>SVTEFLKPRLVDIEQVSSTHAKVTLEPLERGFGHTLGNALRRILLSSMPGCAVTEVEIDGVLHEYSTKEGVQEDILEILLNLKGLAVRVQGKDEVILTLNKSGIGPVTAADITHDGDVEIVKPQHVICHLTDENASISMRIKVQRGRGYVPASTRIHSEEDERPIGRLLVDACYSPVERIAYNVEAARVEQRTDLDKLVIEMETNGTIDPEEAIRRAATILAEQLEAFVDLRDVRQPEVKEEKPEFDPILLRPVDDLELTVRSANCLKAEAIHYIGDLVQRTEVELLKTPNLGKKSLTEIKDVLASRGLSLGMRLENWPPA[2x];> MVYSYTEKKRIRKDFGKRPQVLDVPYLLSIQLDSFQKFIEQDPEGQYGLEAAFRSVFPIQSYSGNSELQYVSYRLGEPVFDVQECQIRGVTYSAPLRVKLRLVIYEREAPEGTVKDIKEQEVYMGEIPLMTDNGTFVINGTERVIVSQLHRSPGVFFDSDKGKTHSSGKVLYNARIIPYRGSWLDFEFDPKDNLFVRIDRRRKLPATIILRALNYTTEQILDLFFEKVIFEIRDNKLQMELVPERLRGETASFDIEANGKVYVEKGRRITARHIRQLEKDDVKLIEVPVEYIAGKVVAKDYIDESTGELICAANMELSLDLLAKLSQSGHKRIETLFTNDLDHGPYISETLRVDPTNDRLSALVEIYRMMRPGEPPTREAAESLFENLFFSEDRYDLSAVGRMKFNRSLLREEIEGSGILSKDDIIDVMKKLIDIRNGKGEVDDIDHLGNRRIRSVGEMAENQFRVGLVRVERAVKERLSLGDLDTLMPQDMINAKPISAAVKEFFGSSQLSQFMDQNNPLSEITHKRRISALGPGGLTRERAGFEVRDVHPTHYGRVCPIETPEGPNIGLINSLSVYAQTNEYGFLETPYRKVTDGVVTDEIHYLSAIEEGNYVIAQANSNLDEEGHFVEDLVTCRSKGESSLFSRDQVDYMDVSTQQVVSVGASLIPFLEHDDANRALMGANMQRQAVPTLRADKPLVGTGMERAVAVDSGVTAVAKRGGVVQYVDASRIVIKVNEDEMYPGEAGIDIYNLTKYTRSNQNTCINQMPCVSLGEPVERGDVLADGPSTDLGELALGQNMRVAFMPWNGYNFEDSILVSERVVQEDRFTTIHIQELACVSRDTKLGPEEITADIPNVGEAALSKLDESGIVYIGAEVTGGDILVGKVTPKGETQLTPEEKLLRAIFGEKASDVKDSSLRVPNGVSGTVIDVQVFTRDGVEKDKRALEIEEMQLKQAKKDLSEELQILEAGLFSRIRAVLVAGGVEAEKLDKLPRDRWLELGLTDEEKQNQLEQLAEQYDELKHEFEKKLEAKRRKITQGDDLAPGVLKIVKVYLAVKRRIQPGDKMAGRHGNKGVISKINPIEDMPYDENGTPVDIVLNPLGVPSRMNIGQILETHLGMAAKGIGDKINAMLKQQQEVAKLREFIQRAYDLGADVRQKVDLSTFSDEEVMRLAENLRKGMPIATPVFDGAKEAEIKELLKLGDLPTSGQIRLYDGRTGEQFERPVTVGYMYMLKLNHLVDDKMHARSTGSYSLVTQQPLGGKAQFGGQRFGEMEVWALEAYGAAYTLQEMLTVKSDDVNGRTKMYKNIVDGNHQMEPGMPESFNVLLKEIRSLGINIELED;> LLKFLKAQTKTEEFDAIKIALASPDMIRSWSFGEVKKPETINYRTFKPERDGLFCARIFGPVKDYECLCGKYKRLKHRGVICEKCGVEVTQTKVRRERMGHIELASPTAHIWFLKSLPSRIGLLLDMPLRDIERVLYFESYVVIEGGMTNLERQQILTEEQYLDALEEFGDEFDAKMGAEAIQALLKSMDLEQECEQLREELNETNSETKRKKLTKRIKLLEAFVQSGNKPEWMILTVLPVLPPDLRPLVPLDGGRFATSDLNDLYRRVINRNNRLKRLLDLAAPDIIVRNEKRMLQEAVDALLDNGRRGRAITGSNKRPLKSLADMIKGKQGRFRQNLLGKRVDYSGRSVITVGPYLRLHQCGLPKKMALELFKPFIYGKLELRGLATTIKAAKKMVEREEAVVWDILDEVIREHPVLLNRAPTLHRLGIQAFEPVLIEGKAIQLHPLVCAAYNADFDGDQMAVHVPLTLEAQLEARALMMSTNNILSPANGEPIIVPSQDVVLGLYYMTRDCVNAKGEGMVLTGPKEAERLYRSGLASLHARVKVRITEYEKDANGELVAKTSLKDTTVGRAILWMIVPKGLPYSIVNQALGKKAISKMLNTCYRILGLKPTVIFADQIMYTGFAYAARSGASVGIDDMVIPEKKHEIISEAEAEVAEIQEQFQSGLVTAGERYNKVIDIWAAANDRVSKAMMDNLQTETVINRDGQEEKQVSFNSIYMMADSGARGSAAQIRQLAGMRGLMAKPDGSIIETPITANFREGLNVLQYFISTHGARKGLADTALKTANSGYLTRRLVDVAQDLVVTEDDCGTHEGIMMTPVIEGGDVKEPLRDRVLGRVTAEDVLKPGTADILVPRNTLLHEQWCDLLEENSVDAVKVRSVVSCDTDFGVCAHCYGRDLARGHIINKGEAIGVIAAQSIGEPGTQLTMRTFHIGGAASRAAAESSIQVKNKGSIKLSNVKSVVNSSGKLVITSRNTELKLIDEFGRTKESYKVPYGAVLAKGDGEQVAGGETVANWDPHTMPVITEVSGFVRFTDMIDGQTITRQTDELTGLSSLVVLDSAERTAGGKDLRPALKIVDAQGNDVLIPGTDMPAQYFLPGKAIVQLEDGVQISSGDTLARIPQESGGTKDITGGLPRVADLFEARRPKEPAILAEISGIVSFGKETKGKRRLVITPVDGSDPYEEMIPKWRQLNVFEGERVERGDVISDGPEAPHDILRLRGVHAVTRYIVNEVQDVYRLQGVKINDKHIEVIVRQMLRKATIVNAGSSDFLEGEQVEYSRVKIANRELEANGKVGATYSRDLLGITKASLATESFISAASFQETTRVLTEAAVAGKRDELRGLKENVIVGRLIPAGTGYAYHQDRMRRRAAG;> ARVTVQDAVEKIGNRFDLVLVAARRARQMQVGGKDPLVPEENDKTTVIALREIEEGLINNQILDVRERQEQQEQ;> AGTPSGNGVGETTQSLQDYLMWQVELTPFTDTDRAIATSIVDAVDDTGYLTIQIEDIVDSIGDDEIGLEEVEAVLKRIQRFDPVGVAAKDLRDCLLIQLSQFAKETPWLEEARLIISDHLDLLANHDFRTLMRVTRLKEEVLKEAVNLIQSLDPRPGQSIQTGEPEYVIPDVLVRKVNDRWVVELNSDSLPSANDTLLRVSRCIVEQQQAFFEQGEEYMKPMVLADIAQAVEMHESTISRVTTQKYLHSPRGIFELKYFFSSHVNTEGGGEASSTAIRALVKKLIAAENPAKPLSDSKLTSMLSEQGIMVARRTVAKYRESLSIPPSNQ

Transcription initiation in bacteria involves the recruitment of RNAP by sigma factors (σ) to promoter regions located upstream from the transcription start site (TSS, position +1). In approximately 60% of bacteria, a major variant σ factor, σ54, forms a class of its own, lacking structural and sequence similarity to σ70. In σ54-mediated transcription initiation, σ54 recruits RNAP to genes responsible for regulating a variety of stress responses, including nutrient depletion, membrane stress, antibiotic exposure, and biofilm formation. In this study, we used single-particle cryo-electron microscopy (cryoEM) to determine the structures of initial transcribing complexes of increasing RNA lengths from 5 nt to 9 nt, which allow us to propose a mechanism of RNAP promoter escape in the σ54 system.

In 8 and 9 nt complexes, the density for the RII-finger is partially lost, indicating this region becoming dynamic in nature and the interactions observed in 7 nt are lost. In addition, P110 and Y112, observed in 5 to 7nt complexes, were also not resolved, indicating that these interactions are no longer stably maintained. Further RNA extension releases RII-finger by breaking the hydrophobic interactions between the β′ lid and RII residues P110 and Y112. At RPitc-8nt and -9nt, both template and nontemplate strands scrunch around the ELH, losing interactions between the DNA strands and ELH, resulting in reduced density for both DNA and the ELH. As RNA length increases to 9 nt, RII becomes more flexible. Our results thus suggest that DNA scrunching is a major mechanism during initial transcription up to 9 nt with progressively more scrunches occurring, initially close to the active site and then move upstream toward the σ54 ELH. Furthermore, we also observe the loss of resolution of the upstream DNA and upstream DNA binding domains on σ54 (RpoN, ELH-HTH), suggesting that both the σ54 upstream DNA binding subdomains and upstream DNA are less stably engaged with RNAP. Interestingly, the proportion of σ54-free complexes increases with increasing RNA lengths, suggesting that the σ54-RNAP complexes become increasingly unstable.Re-annotation of the activity of an earlier enzyme in the pathway, MenD, then led to the recognition that the true enzymatic activity of MenH is to covert the MenD reaction product, 2-succinyl-5-enolpyruvyl-6-hydroxy-3-cyclohexene-1-carboxylate (SEPHCHC) to 2-succinyl-6-hydroxy-2,4-cyclohexadiene-1-carboxylate (SHCHC) by a 2,5 elimination of pyruvate from the cyclohexene ring. MenH is thus correctly annotated as SHCHC synthase. EcMenH adopts a typical α/β-hydrolase fold, comprising a core β-sheet of mostly parallel strands surrounded on both sides by α-helices. As is characteristic of the α/β-hydrolases the three catalytic triad residues (Ser86, His232, Asp210) are located on loops of the core α/β–domain.

Accordingly, we report the structure of the MenH from E. coli at 2.75 Å resolution, along with the structures of two active site mutant enzymes, Arg124Ala and Tyr85Phe, both at 2.5 Å resolution. Structural comparisons of native EcMenH with the two mutant structures, R124A and Y85F using SSM shows they overlay very closely, with rms differences of 0.26–0.61 Å in Cα-atom positions over the entire structure. This shows that the mutations do not affect the polypeptide conformation significantly. In addition, 5–6 residues of the N-terminal His6 tag could be modeled for two of the chains in all the I4122 structures and in all chains of the Tyr85Phe C2 mutant structure. The Tyr85 aromatic ring is packed between the side chains of Ser86 and His235, while its OH group is hydrogen bonded to a water molecule and the catalytic His232 (a C-H…O bond), and interacts with the bound chloride ion (3.1–3.3 Å). For the Y85F mutant, the contact between the succinyl carboxyl group and the phenolic oxygen of Tyr85 is necessarily lost, with the carboxyl group then being positioned closer to Tyr148 OH and Trp147 NE than in the other structures; it is consistently hydrogen bonded to both. In our EcMenH structures, the indole NH of Trp147 and the OH of Tyr85 are ∼7.5 Å apart, well placed to bind the succinyl carboxylate between them, as shown in the docking studies. Mutation of either one of them may not compromise binding, especially as other residues such as Tyr148 and Arg168 could then become involved, but such mutations could compromise productive binding, thereby affecting catalysis. If, as suggested, substrate binding is required before the catalytic triad can become active, Tyr85, which binds to both substrate and His232, could play a key role in activation of catalysis. The structure is not perturbed by the mutations.

>[3x]MHHHHHHSSGLVPRGSMILHAQAKHGKPGLPWLVFLHGFSGDCHEWQEVGEAFADYSRLYVDLPGHGGSAAISVDGFDDVTDLLRKTLVSYNILDFWLVGFSLGGRVAMMAACQGLAGLCGVIVEGGHPGLQNAEQRAERQRSDRQWVQRFLTEPLTAVFADWYQQPVFASLNDDQRRELVALRSNNNGATLAAMLEATSLAVQPDLRANLSARTFAFYYLCGERDSKFRALAAELAADCHVIPRAGHNAHRENPAGVIASLAQILRF> MKGIIFTEFLDLVEDKFGLEMVDKIITQSELESEGVYTSIGTYRFSEMLQLLQNLSANTDVSIDDLLLTYAEHFFSVIEDSYPGLLATYKDPIEMLASIENHIHVEVRKIYPDAELPTFVVEEKTANSLTMIYKSSRAMHHFGLGLMNKTFEHFNSSAEIILEKIK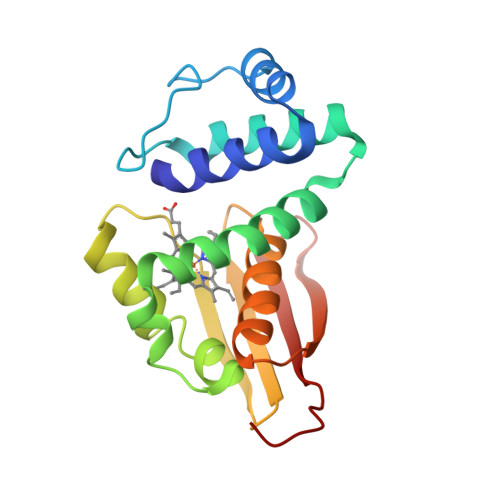EDGTEVKFIINKNENLYFQ> DYKDDDDKLHSQANLMRLKSDLFNRSPMYPGPTKDDPLTVTLGFTLQDIVKADSSTNEVDLVYYEQQRWKLNSLMWDPNEYGNITDFRTSAADIWTPDITAYSSTRPV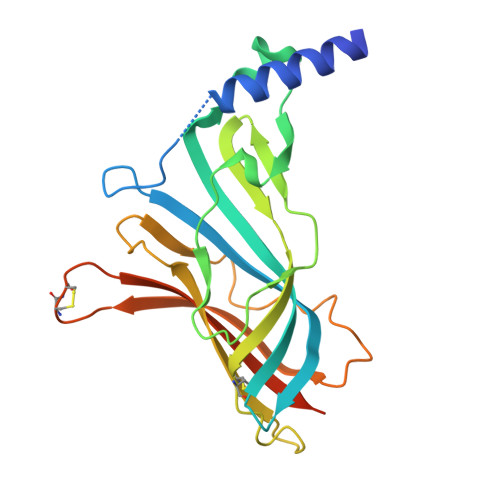QVLSPQIAVVTHDGSVMFIPAQRLSFMCDPTGVDSEEGATCAVKFGSWVYSGFEIDLKTDTDQVDLSSYYASSKYEILSATQTRQVQHYSCCPEPYIDVNLVVKFRERRAGNGFFRNLFDSR> AIASEFSSLPSYAAYATAQEAYEQAVANGDSEVVLKKLKKSLNVAKSEFDRDAAMQRKLEKMADQAMTQMYKQARSEDKRAKVTSAMQTMLFTMLRKLDNDALNNIINNARDGCVPLNIIPLTTAAKLMVVVPDYGTYKNTCDGNTFTYASALWEIQQVVDADS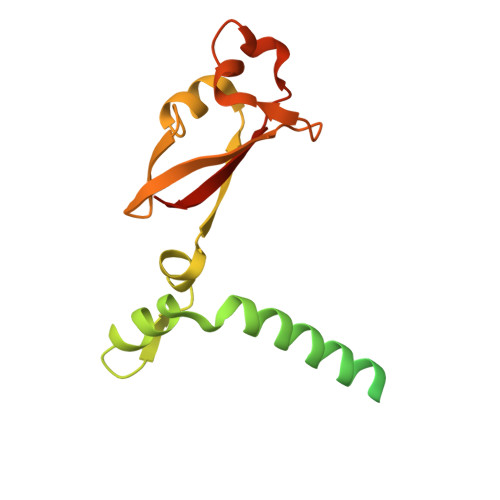KIVQLSEINMDNSPNLAWPLIVTALRANSAVKLQ> MRAGLLEGVIKEKGGVPVYPSYLAGEWGGSGQEIEVKSPIDLATIAKVISPSREEVERTLDVLFKRGRWSARDMPGTERLAVLRKAADIIERNLDVFAEVLVMNAGKPKSAAVGEVKAAVDRLRLAELDLKKIGGDYIPGDWTYDTLETEGLVRREPLGVVAAITPFNYPLFDAVNKITYSFIYGNAVVVKPSISDPLPAAMAVKALLDAGFPPDAIALLNLPGKEAEKIVADDRVAAVSFTGSTEVGERVVKVGGVKQYVMELGGGDPAIVLEDADLDLAADKIARGIYSYAGQRCDAIKLVLAERPVYGKLVEEVAKRLSSLRVGDPRDPTVDVGPLISPSAVDEMMAAIEDAVEKGGRVLAGGRRLGPTYVQPTLVEAPADRVKDMVLYKREVFAPVALAVEVKDLDQAIELANGRPYGLDAAVFGRDVVKIRRAVRLLEVGAIYINDMPRHGIGYYPFGGRKKSGVFREGIGYAVEAVTAYKTIVFNYKGKGV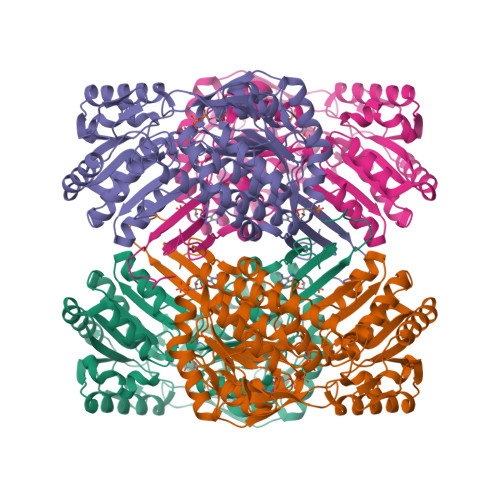WKYE>DEPNQPSTPEAVTKTVTIDASKYETWQYFSFSKGEVVNVTDYKNDLNWDMALHRYDVRLNCGESGKGKGGAVFSGKTEMDQATTVPTDGYTVDVLGRITVKYE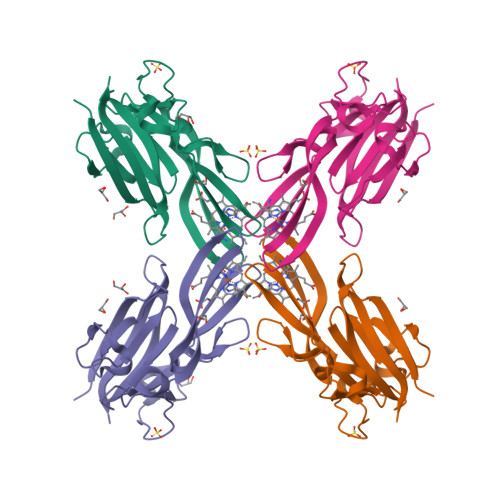MGPDGHQMEYEEQGFSEVITGKKNAQGFASGGWLEFSHGPAGPTYKLSKRVFFVRGADGNIAKVQFTDYQDAELKKGVITFTYTYPVK[2x]>[4x]GSNLAAWKISIPYVDFFEDPSSERKEKKERIPVFCIDVERNDRRAVGHEPEHWSVYRRYLEFYVLESKLTEFHGAFPDAQLPSKRIIGPKNYEFLKSKREEF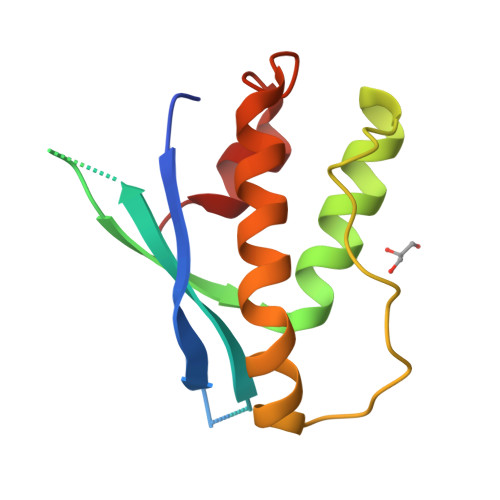QEYLQKLLQHPELSNSQLLADFLSPN Sister chromatid cohesion is mediated by cohesin, whose Smc1, Smc3, and kleisin (Scc1) subunits form a ring structure that entraps sister DNAs. The ring is opened either by separase, which cleaves Scc1 during anaphase, or by a releasing activity involving Wapl, Scc3, and Pds5, which bind to Scc1 and open its interface with Smc3. We present crystal structures of Pds5 from the yeast L. thermotolerans in the presence and absence of the conserved Scc1 region that interacts with Pds5. Thus, Pds5 can be considered the gatekeeper of the cohesin ring.

The region within kleisin Scc1 of cohesin that binds Pds5 has been mapped previously (Chan et al., 2013), and we therefore synthesized a 23-amino-acid-long peptide from L. thermotolerans Scc1 (121–143) containing this region. Although binding was weak (Chan et al., 2013), molecular replacement and a difference Fourier map with data collected from co-crystals of LtPds5 containing the LtScc1 peptide revealed clear difference density. We could locate and model residues 125–141 of Scc1 in the density, using data from two SeMet single-wavelength anomalous diffraction (SAD) datasets from crystals with Scc1 peptides containing SeMet residues to confirm the sequence assignment (red and green densities). Molecular replacement with four fragments was required because Pds5 shows changes in conformation upon peptide binding. The hook opens and the entire structure bends such that the most N-terminal part (left, top) moves by up to 10 Å relative to the central part (superposition based on Cα atoms of residues 473 to 726). The nose becomes disordered in the co-crystals. In the Pds5:Scc1 complex structure, the Pds5 hook opens because the Scc1 peptide is wedged between the spine and the end of the hook, maintaining a closed-ring architecture (bottom). Acidic and hydrophobic residues that in the apo structure of Pds5 make the contact with the spine, D999, M1027 and Y1031, now interact with the Scc1 peptide. In the complex, Scc1 is in a mostly extended conformation, except toward its C terminus, which forms a more compact arrangement with helical turns. In contrast, other mutations, namely, ScScc1 L126K, L128E, V132K, T133K, E134K, and E136K, had little or no effect (corresponding to Lt L128K, L129E, V133K, T134K, E135K, and E137K). As is indicated in Figure 1D, Scc1 V138 sits in a deep pocket in Pds5, lined by Pds5 Y493 and other hydrophobic residues.

> XXXXXXXXXXXXXXXXXXXXXXXXXXXXXXXXXXXXXXXXXXXXXLERYRADLIDRKILRNKDHGVRAFAACCLSDILRLYAPDAPYTDKELTEIFRLFLAQLKLLQEPENGYLTQQTYLINNLLEYRSIVILTDLPSSSQLVEELFNIFYSPTNSTIQGNMFTAIGGILGEVISECDSLPMSALKMVFNKFLSHKRAESLDGINYKKDPGFEISLIICQTYSNRLGRHFIKFYSEIMYEVLGESDIHEKGIASSAYKTLVKIGNLTSELWKYAPELVGSVTGLLYQLLCSDNELFRESATKCVSKMLGTHSLINFAVAHSDTYKIWLSKMADISPHVRQAWVSEIPSILMSRSDLSDDISKGLAKALIDSDHTVRLSAIQTFHEVPVKRLWECLPNAAVFAGLVHLTRETRRDLRDECIDAVARIYTESIESIPKTNENKEIWGVVETIPSACFNLYYINDLEINMKVDLLTFEKFLPLGLSNEEFVQRLLTLLQGFNEKAFSSFYAFNRRQDQMSTVLWKFIEFCEETNSQSPAASLSDTKLIKTVEWISSGFPSHLNVEQILLAFRELNDRRLYRLIKVAVAETSKHLTVRNAVSELFKRLEEPELFRKKNIKIESRFTRDNFSTVFRVLIYRAAPIIFNISNLPSFLNTSDSSNEDEKALKRQLIDNISIIKPGIFKDQVKNLVTIITEGETTGPGNTLSLAEAMRTVYKISKDKREHLDIEENTFFFQKLEDYAKEGNPLEAKYAIKLLGLAPNAAEYLSEVATAILPLDLKSKHFASNVLVLAEITKMQPQLLEKDSTEIVGLLIKDVLLSNDVVGDEDDQQAWFSDEDIYTGKADALSAKVFSLKLFANKIKVMAPDAHADEMTHAFTERTLKLFFYLVASGGELVSESNTDNYPTPANYQNKLRCCAGLHILKITKIASLSRFIKPQDISKLMNLVEDESLEVRSSFIGRLKDFLGDGSISIKFLPLVFFTAYEPDQALRTSTKMWINYTLSKENFRKGTFFERALPRLIHFIAHHPDVAEGLRLRETAFLTGLTTAIDYLVFYADSVLKASNLALLYYLAGRVRQYXXXXXXXXXXXXXXXXXXXXXXXXXXXXXXXXXXXXXXXXXXXXXXXXXXXXXXXXXX;> LTNPSQYLLQDAVTEREVLLVP>MVLKERQDGVLVLTLNRPEKLNAITGELLDALYAALKEGEEDREVRALLLTGAGRAFSAGQDLTEFGDRKPDYEAHLRRYNRVVEALSGLEKPLVVAVNGVAAGAGMSLAL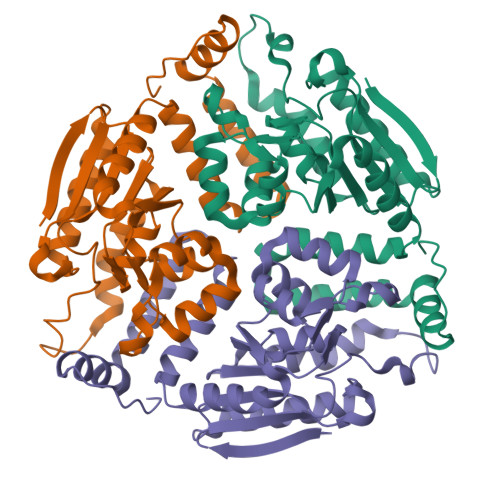WGDLRLAAVGASFTTAFVRIGLVPDSGLSFLLPRLVGLAKAQELLLLSPRLSAEEALALGLVHRVVPAEKLMEEALSLAKELAQGPTRAYALTKKLLLETYRLSLTEALALEAVLQGQAGQTQDHEEGVRAFREKRPPRFQGR[6x]>[4x]PVPNPTMPVKGAGTTLWVYKGSGDPY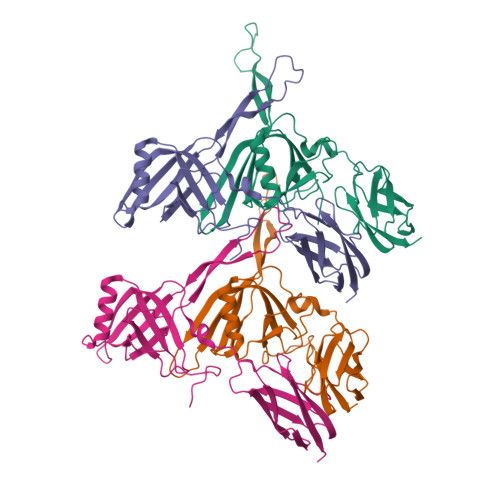ANPLSDVDWSRLAKVKDLTPGELTAESYDDSYLDDEDADWTATGQGQKSAGDTSFTLAWMPGEQGQQALLAWFNEGDTRAYKIRFPNGTVDVFRGWVSSIGKAVTAKEVITRTVKVTNVGRPSMAEDRSTVTAATGMTVTPASTSVVKGQSTTLTVAFQPEGVTDKSFRAVSADKTKATVSVSGMTITVNGVAAGKVNIPVVSGNGEFAAVAEITVTAS>MRGSHHHHHHGSMTDTYLHETLVFDNKLSYIDNQRDTDGPAILLLPGWCHDHRVYKYLIQELDADFRVIVPNWRGHGLSPSEVPDFGYQEQVKDALEILDQLGVETFLPVSHAHGGWVLVELLEQAGPERAPRGIIMDWLMWAPKPDFAKSLTLLKDPERWREGTHGLFDVWLDGHDEKRVRHHLLEEMAD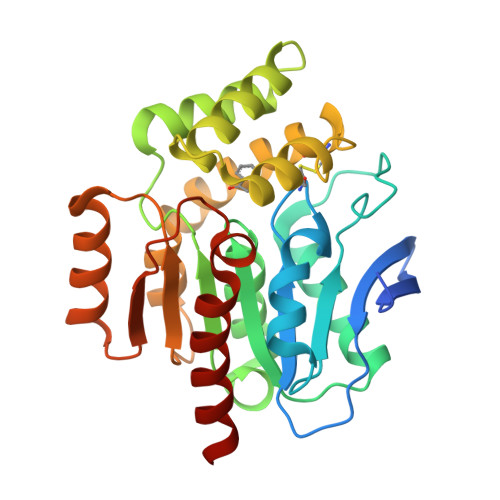YGYDCWGRSGRVIEDAYGRNGSPMQMMANLTKTRPIRHIFSQPTEPEYEKINSDFAEQHPWFSYAKLGGPTHFPAIDVPDRAAVHIREFATAIRQGQ[4x]> CGCAAAAAAGCG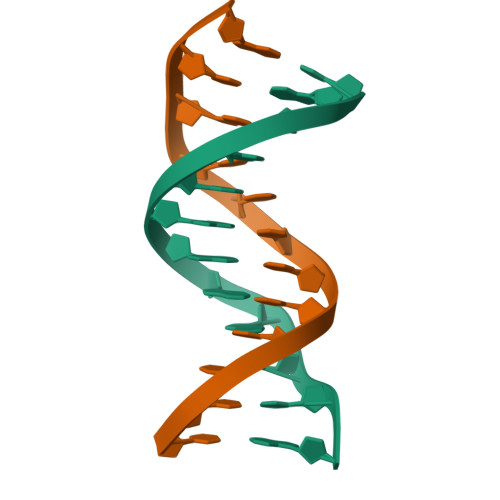;> CGCTTTTTXGCG>[16x]AGADEERAETARLSSFIGAIAIGDLVKSTLGPKGMDKILLSSGRDASLMVTNDGATILKNIGVDNPAAKVLVDMSRVQDDEVGDGTTSVTVLAA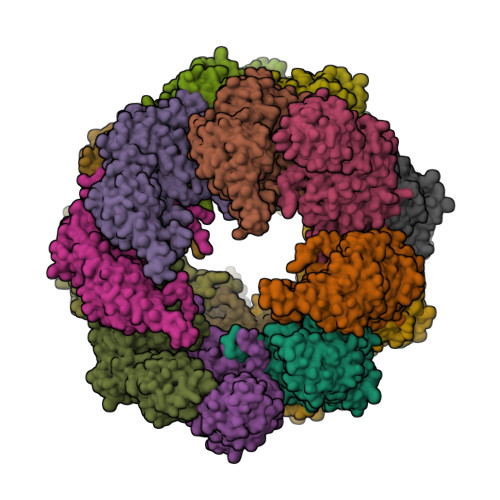ELLREAESLIAKKIHPQTIIAGWREATKAARQALLNSAVDHGSDEVKFRQDLMNIAGTTLSSKLLTHHKDHFTKLAVEAVLRLKGSGNLEAIHVIKKLGGSLADSYLDEGFLLDKKIGVNQPKRIENAKILIANTGMDTDKIKIFGSRVRVDSTAKVAEIEHAEKEKMKEKVERILKHGINCFINRQLIYNYPEQLFGAAGVMAIEHADFVGVERLALVTGGEIASTFDHPELVKLGSCKLIEEVMIGEDKLIHFSGVALGEACTIVLRGATQQILDEAERSLHDALCVLAQTVKDSRTVYGGGCSEMLMAHAVTQLASRTPGKEAVAMESYAKALRMLPTIIADNAGYDSADLVAQLRAAHSEGKTTAGLDMKEGTIGDMSVLGITESFQVKRQVLLSAAEAAEVILRVDNIIKAAPR>[3x]HHHHHHGLIQERRSHEVNPAAHLTGANSSLTGSGGPLLWETQLGLAFLRGLSYHDGALVVTKAGYYYIYSKVQLGGVGCPLGLASTITHGLYKRTPRYPEELELLVSQQSPCGRATSSSRVWWDSSFLGGVVHLEAGEEVVVRVLDERLVRLRDGTRSYFGAFMV;>INITSSASQEGTRLNLICTVWHKKEEAEGFVVFLCKDRSGDCSPETSLKQLR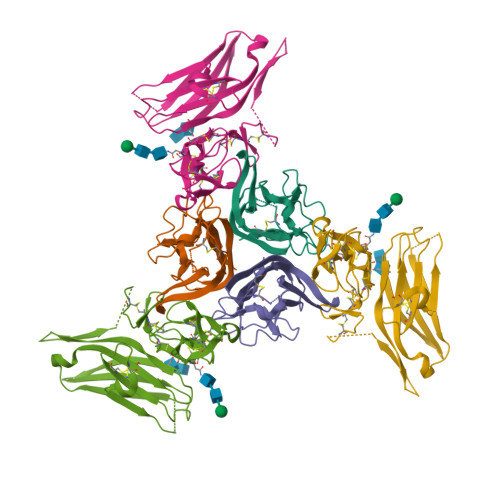LKRDPGIDGVGEISSQLMFTISQVTPLHSGTYQCCARSQKSGIRLQGHFFSILFTETGNYTVTGLKGGGGSGGGGSGGGGSGGGGSLPSCKEDEYPVGSECCPKCSPGYRVKEACGELTGTVCEPCPPGTYIAHLNGLSKCLQCQMCDPAMGLRASRNCSRTENAVCGCSPGHFCIVQDGDHCAACRAYATGHHHHHH[3x]>[4x]GPAESLPD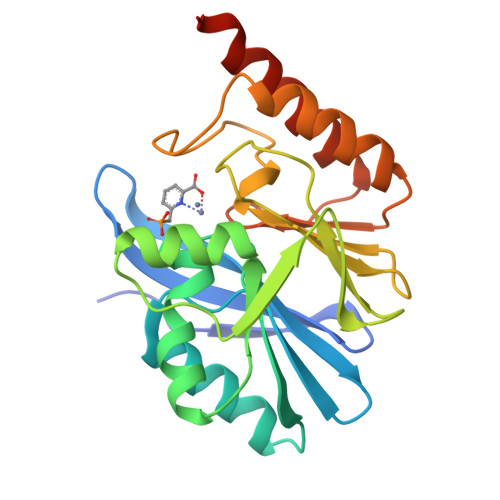LKIEKLDEGVYVHTSFEEVNGWGVVPKHGLVVLVNAEAYLIDTPFTAKDTEKLVTWFVERGYKIKGSISSHFHSDSTGGIEWLNSRSIPTYASELTNELLKKDGKVQATNSFSGVNYWLVKNKIEVFYPGPGHTPDNVVVWLPERKILFGGCFIKPYGLGNLGDANIEAWPKSAKLLKSKYGKAKLVVPSHSEVGDASLLKLTLEQAVKGLNESKKPSNPSN> GASAPMVKIYTKNGDKGQTRIIGKQILYKNDPRVAAYGEVDELNSWVGYTKSLINSHTQVLSNELEEIQQLLFDCGHDLATPADDERHSFKFKQEQPTVWLEEKIDNYTQVVPAVKKAILPGGTQLASALHVARTITRRAERQIVQLMREEQINQDVLIFINRLSDYFFAAARYANYLEQQPD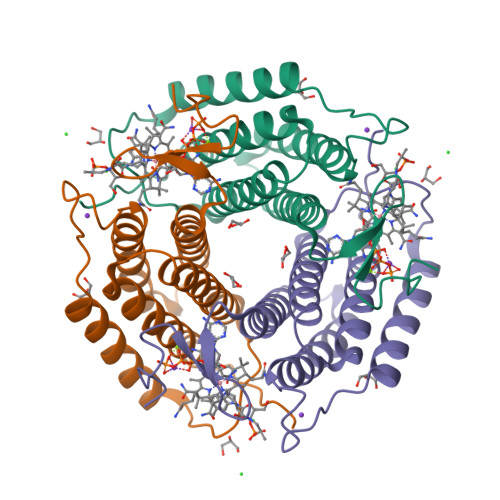MLYRNSKDVFR> MGSSHHHHHHENLYFQSNAAIASEFSSLPSYAAFATAQEAYEQAVANGDSEVVLKKLKKSLNVAKSEFDRDAAMQRKLEKMADQAMTQMYKQARSEDKRAKVTSAMQTMLFTMLRKLDNDALNNIINNARDGCVPLNIIPLTTAAKLMVVIPDYNTYKNTCDGTTFTYASALWEIQQVVDADSKIVQLSEISMDNSPNLAWPL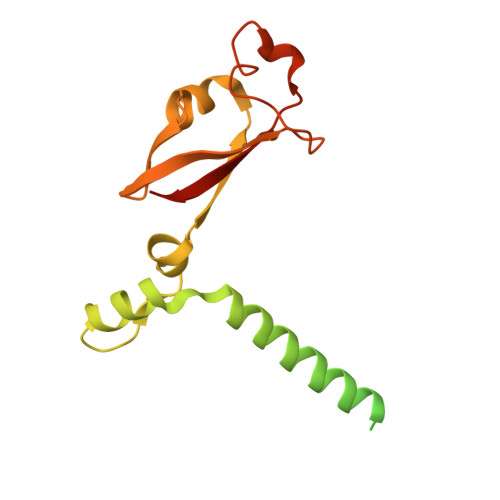IVTALRANSAVKLQ>[2x]TPAFNKPKVELHVHLDGAIKPE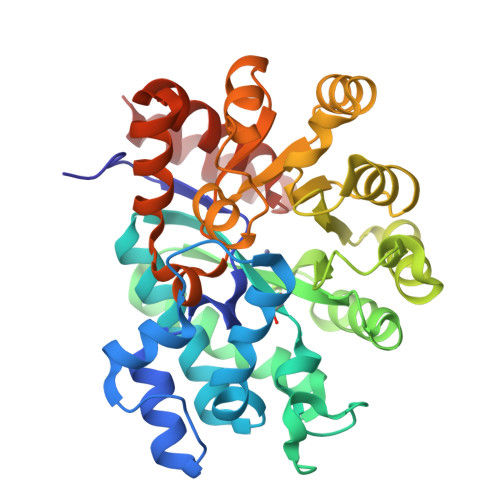TILYFGKKRGIALPADTVEELRNIIGMDKPLSLPGFLAKFDYYMPVIAGCREAIKRIAYEFVEMKAKEGVVYVEVRYSPHLLANSKVDPMPWNQTEGDVTPDDVVDLVNQGLQEGEQAFGIKVRSILCCMRHQPSWSLEVLELCKKYNQKTVVAMDLAGDETIEGSSLFPGHVEAYEGAVKNGIHRTVHAGEVGSPEVVREAVDILKTERVGHGYHTIEDEALYNRLLKENMHFEVCPWSSYLTGAWDPKTTHAVVRFKNDKANYSLNTDDPLIFKSTLDTDYQMTKKDMGFTEEEFKRLNINAAKSSFLPEEEKKELLERLYREYQ> MIVYNNQAPDAVNNVGQFGATEGSIGAYKQAAEYAADSKYWALLAESKFGTIDDLIAEVERLYQQGVLMKQDIEDLKQDFKDQDARLMSLIAQTNAAVSDANNAVALINQKLIEVQNQLDVLLGMSVDVTTLPPGTPATGSFNPNTGVISLGIPEGEPGKDGSVKDLDTAPTGVPELGDLGFYVDKDDNTVHKTTLENIANLTPSVRSVSVNGGPALDGEVALTINKETVGLGNVLNVAQYSRQEINDKFDKTTKTYQSKAEAYADAQYRQVGEKVLVWEATKYEFYTVAANKTLTPVKTEGRILTVNSRSPDSSGNIDITIPTGNPSLYLGEMVMFPYDPSKNISYPGVLPADGRLVSKESASDLGPSLVSGQLPVVSETEWQSGAKQYFSWGKLADGITDADSTNFINIRLPDWTGGEAIRAPDSDKDSQYNGSVQAQKPYVVTVNNQAPDEITGNVNISRSILGAASSGANSDITSLSGLTTPLSISQGGTGAKDAASARSNLGLGSVSTLDNVPIASGGTGAGDAAGARFNLGLGNSATMNTGTNSDNVLKVGDFGIGRPDGALVFDTTSQDQLLAGLDTYGLCVFRNNQQIAAPWDIWNYSSNLFFRAGDTYSMISIPFESAGKIKVFGGASGSGWKTSRTVYDTVNTTVDVNGFIKAASPIVKVFHDGSFETNEQSDGVSVKKISTGVYLISGCLGLNSDAGWGGVDGGFEIPIDRNKQPRVWLDYEVKEDGSLL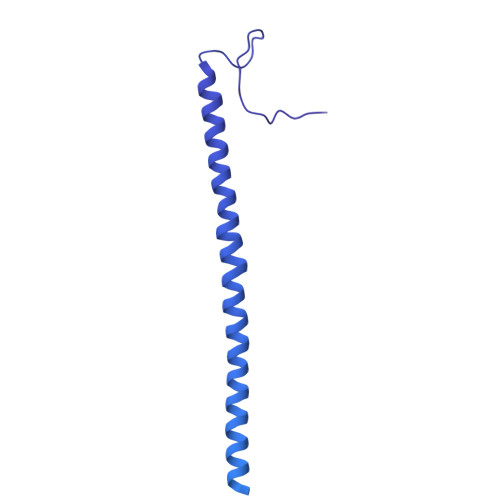IKTYHRTHSTSPAFARNELEGFSDGDPVDIPKDAFISVRVEMPSK> ETGTVPAINYLGAGYDHVRGNPVGDPSSMGDPGIRPPVLRFTYAQNEDGVSNDLTVLQPLGGYVRQYVACRQSETISELSNLSDYQNELSVDASLQGGDPIGLNSFSASTGYRDFAKEVSKKDTRTYMLKNYCMRYEAGVAQSNHFKWNVTLAFAA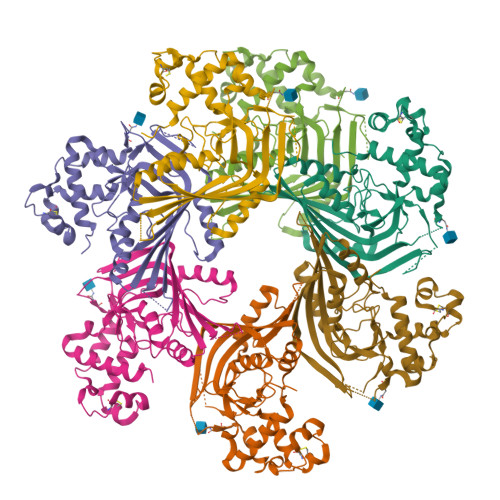GVSQLPDVFDAHNPECACSAEQWRQDQNAEACTKTNVPIWISFIEQFGTHFLVRLFAGGKMTYQVTAKRSEVEKMRNMGIDVKTQLKMQLGGVSGGAGQGTSSKKQQSSSEYQMNVQKETLVIGGRPPGQVSDPAALAAWADTVEELPMPVKFEVQPLYHLLPVEKQEAFKQAVTFYSKAVGLTPQDLSALGTKHHHHHH> MTFVRELRSRTFDSSDEVILKPTGNQLTVEFLEENSFSVPILVLKKDGLGMTLPSPSFTVRDVEHYVGSDKEIDVIDVTRQADCKMKLGDFVKYYYSGKREKVLNVISLEFSDTRLSNLVETPKIVRKLSWVENLWPEECVFERPNVQKYCLMSVRDSYTDFHIDFGGTSVWYHVLKGEKIFYLIRPTNANLTLFECWSSSSNQNEMFFGDQVDKCYKCSVKQGQTLFIPTGWIHAVLTPVDCLAFGGNFLHS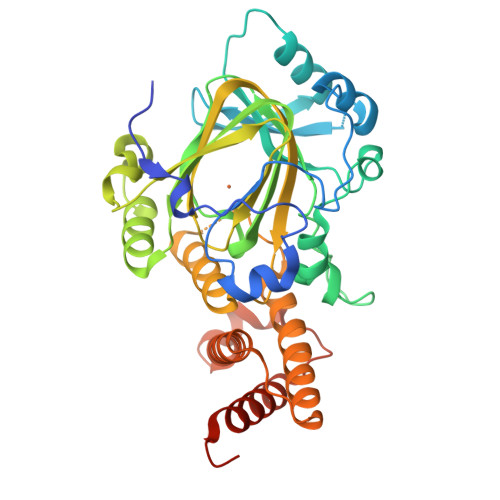LNIEMQLKAYEIEKRLSTADLFRFPNFETICWYVGKHILDIFRGLRENRRHPASYLVHGGKALNLAFRAWTRKEALPDHEDEIPETVRTVQLIKDLAREIRLVEDIFQQNLEHHHHHH> G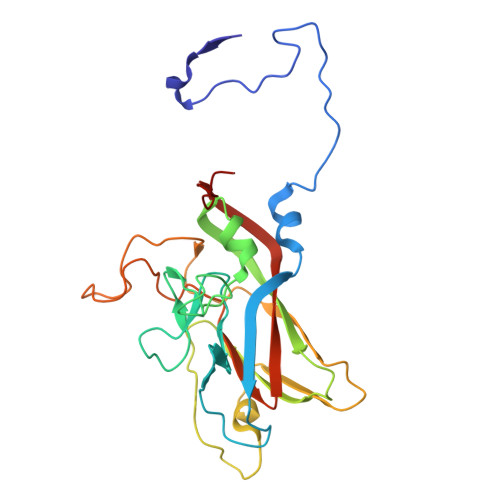VDNAEKGKVSDDNASTDFVAEPVKLPENQTRVSFFYDRSTLSSVLQSTSDVSSKFTPSTAKNLQNSILLTPLPSDIVNNSVLPEQERWISFASPTTQKPPYKTKQDWNFIMFSPFTYYKCDLEVTLSKNDRETISSVVRYVPCGAPSDLSDQTMPQTPSLADTRDPHMWVVGQGTTNQISFVIPYTSPLSVLPSVWFNGFSNFDNSSRFGVAPNADFGRLLLQGQGTFSVHYRYKKMRVFCPRPTVFIPWP>FPVATNGERFPWQELRLPSVVIPLHYDLFVHPNLTSLDFVASEKIEVLVSNATQFIILHSKDLEITNATLQSEEDSRYMKPGKELKVLSYPAHEQIALLVPEKLTPHLKYYVAMDFQAKLGDGFEGFYKSTYRTLGGETRILAVTDFEPTQARMAFPCFDEPLFKANFSIKIRRESRHIALSNMPKVKTIELEGGLLEDHFETTVKMSTYLVAYIVCDFHSLSGFTSSGVKVSIYASPDKRNQTHYALQASLKLLDFYEKYFDIYYPLSKLDLIAIPDFAPGAMENWGLITYRETSLLFDPKTSSASDKLWVTRVIAHELAHQWFGNLVTMEWWNDIWLNEGFAKYMELIAVNATYPELQFDDYFLNVCFEVITKDSLNSSRPISKPAETPTQIQEMFDEVSYNKGACILNMLKDFLGEEKFQKGIIQYLKKFSYRNAKNDDLWSSLSNSCLESDFTSGGVCHSDPKMTSNMLAFLGENAEVKEMMTTWTLQKGIPLLVVKQDGCSLRLQQERFLQGVFQEDPEWRALQERYLWHIPLTYSTSSSNVIHRHILKSKTDTLDLPEKTSWVKFNVDSNGYYIVHYEGHGWDQLITQLNQNHTLLRPKDRVGLIHDVFQLVGAGRLTLDKALDMTYYLQHETSSPALLEGLSYLESFYHMMDRRNISDISENLKRYLLQYFKPVIDRQSWSDKGSVWDRMLRSALLKLACDLNHAPCIQKAAELFSQWMESSGKLNIPTDVLKIVYSVGAQTTAGWNYLLEQYELSMSSAEQNKILYALSTSKHQEKLLKLIELGMEGKVIKTQNLAALLHAIARRPKGQQLAWDFVRENW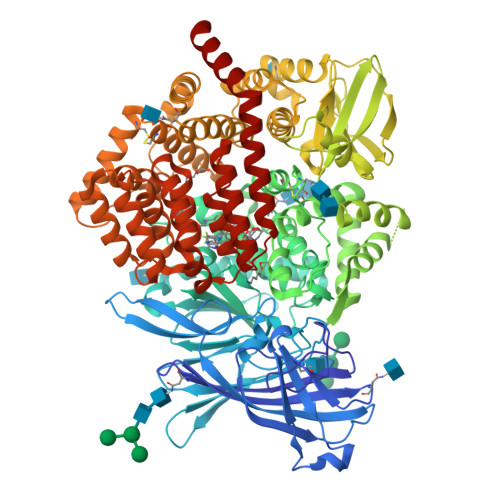THLLKKFDLGSYDIRMIISGTTAHFSSKDKLQEVKLFFESLEAQGSHLDIFQTVLETITKNIKWLEKNLPTLRTWLMVNTRHH[2x]> MSMLKREDWYDLTRTTNWTPKYVTENELFPEEMSGARGISMEAWEKYDEPYKITYPEYVSIQREKDSGAYSIKAALERDGFVDRADPGWVSTMQLHFGAAALEEYAASTAEARMARFAKAPGNRNMATFGMMDENRHGQIQLYFPYANVKRSRKWDWAHKAIHTNEWAAIAARSFFDDMMMTRDSVAVSIMLTFAFETGFSNMQFLGLAADAAEAGDHTFASLISSIQTDESRHAQQGGPSLKILVENGKKDEAQQMVDVAIWRSWKLFSVLTGPIMDYYTPLESRNQSFKEFMLEWIVAQFERQLLDLGLDKPWYWDQFMQDLDETHHGMHLGVWYWRPTVWWDPAAGVSPEEREWLEEK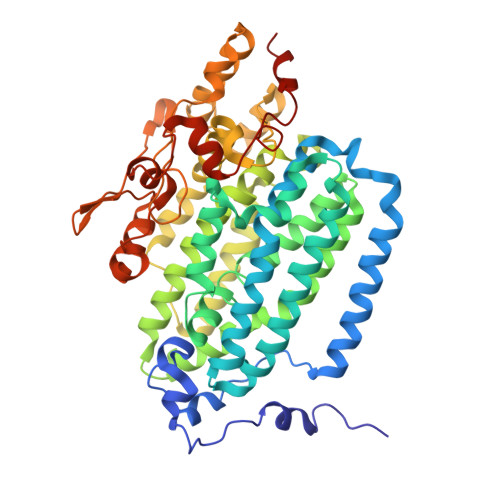YPGWNDTWGQCWDVITDNLVNGKPELTVPETLPTICNMCNLPIAHTPGNKWNVKDYQLEYEGRLYHFGSEADRWCFQIDPERYKNHTNLVDRFLKGEIQPADLAGALMYMSLEPGVMGDDAHDYEWVKAYQKKTNAA> SNGLFGANTLSNMGKDTILRFQMFTKWKANGYLPKKIKDDIPRSL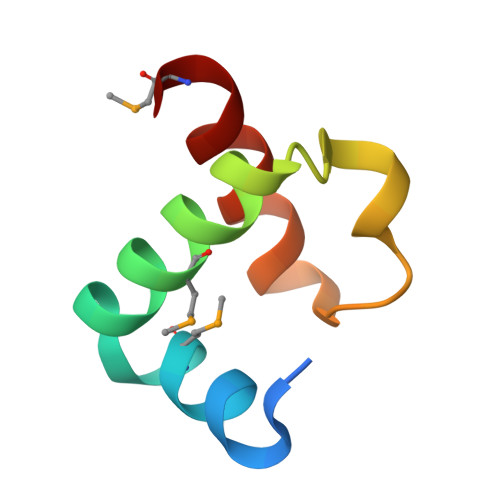YKAYKIHYRMN> RKSRITNYPKLEDANKAGTKEGYKCTLVLTEGDSALSLAVAGLAVVGRDYYGCYPLRGKMLNVREASADQILKNAEIQAIKKIMGLQHRKKYEDTKSLRYGHLMIMTDQDHDGSHIKGLIINFLESSFLGLLDIQGFLLEFITPIIKVSITKPTKNTIAFYNMPDYEKWREEESHKFTWKQKYYKGLGTSLAQEVREYFSNLDRHLKIFHSLQGNDKDYIDLAFSKKKADDRKEWLRQYEPGTVLDPTLKEIPISDFINKELILFSLADNIRSIPNVLDGFKPGQRKVLYGCFKKNLKSELKVAQLAPYVSECTAYHHGEQSLAQTIIGLAQNFVGSNNIYLLLPNGAFGTRATGGKDAAAARYIYTELNKLTRKIFHPADDPLYKYIQEDEKTVEPEWYLPILPMILVNGAEGIGTGWSTYIPPFNPLEIIKNIRHLMNDEELEQMHPWFRGWTGTIEEIEPLRYRMYGRIEQIGDNVLEITELPARTWTSTIKEYLLLGLSGNDKIKPWIKDMEEQHDDNIKFIITLSPEEMAKTRKIGFYERFKLISPISLMNMVAFDPHGKIKKYNSVNEILSEFYYVRLEYYQKRKDHMSERLQWEVEKYSFQVKFIKMIIEKELTVTNKPRNAIIQELENLGFPRFNKEGKPYYGSPNDEIAEQINDVKGATSDEEDEESSH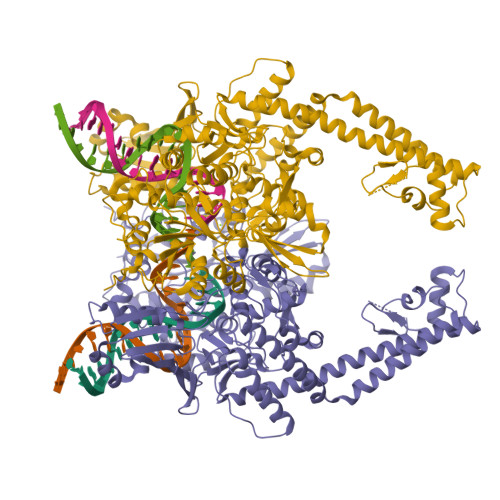EDTENVINGPEELYGTYEYLLGMRIWSLTKERYQKLLKQKQEKETELENLLKLSAKDIWNTDLKAFEVGYQEFLQRDAEAR> 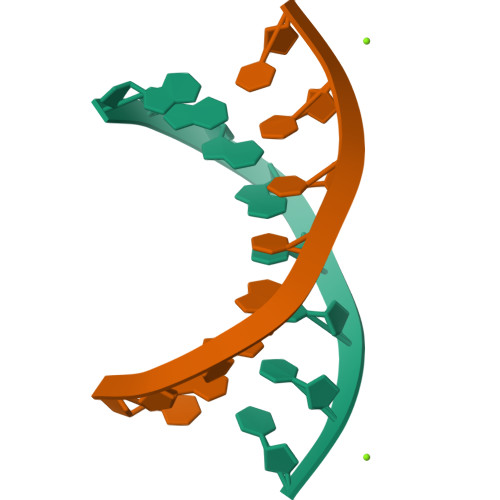GAGGCCTC>MFGRAPMKAATATAAVGFSCLCYHTLPHLRYPAELPTLGFNYKDGIQPVMSPRQLELHYSKHHSAYVDKLNTLGKGYEGKTIEEIILATTGINESKVMFNQAAQHFNHSFFWKCLSPGGKPMPKTLENAI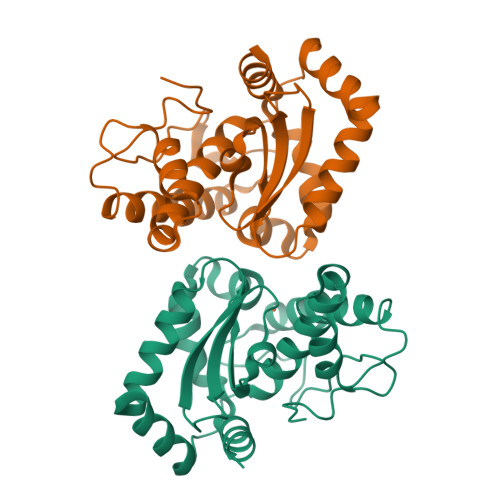AKQFGSVDDFMVSFQQAGVNNFGSGWTWLCVDPQTKELLIDSTSNAGCPLTSGLRPIFTADVWEHAYYKDFENRRADYLKELWQIVDWEFVCHMYERATK[12x]1-methoxy-4-oxoquinoline 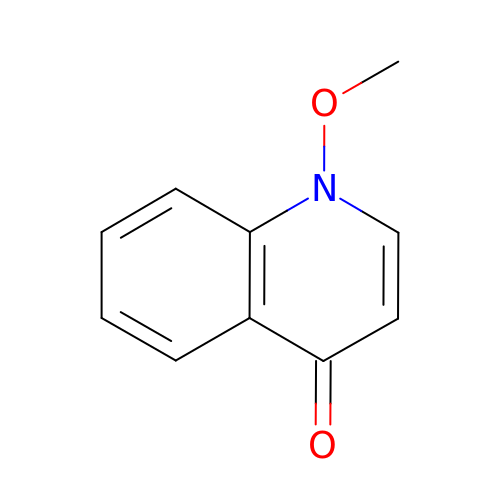| C10 H9 N O2 | QKCKRWUYZIGMET-UHFFFAOYSA-N> GGATAGCTAGGA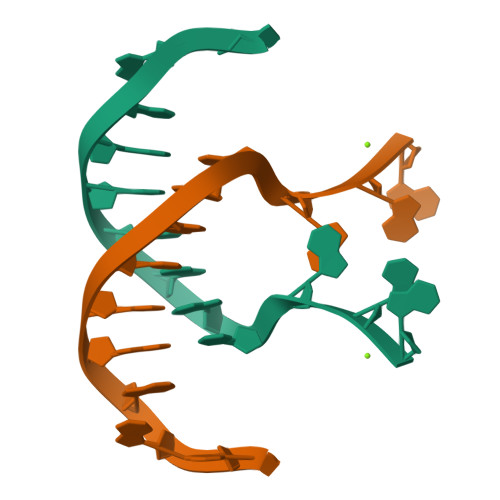G>[6x]MNDLEKKFYELPELPYPYDALEPHISREQLTIHHQKHHQAYVDGANALLRKLDEARESDTDVDIKAALKELSFHVGGYVLHLFFWGNMGPADECGGEPSGKLAEYIEKDF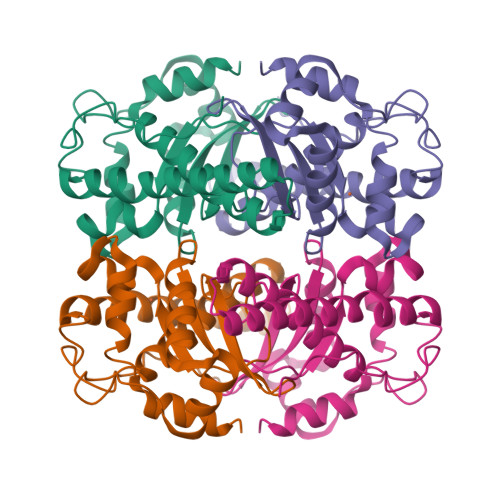GSFERFRKEFSQAAISAEGSGWAVLTYCQRTDRLFIMQVEKHNVNVIPHFRILLVLDVWEHAYYIDYRNVRPDYVEAFWNIVNWKEVEKRFEDIL> MWRKLLNNHHDDASKFICLLAKPNCSSLEQEDFIPLLQDVVDTHPGLTFLK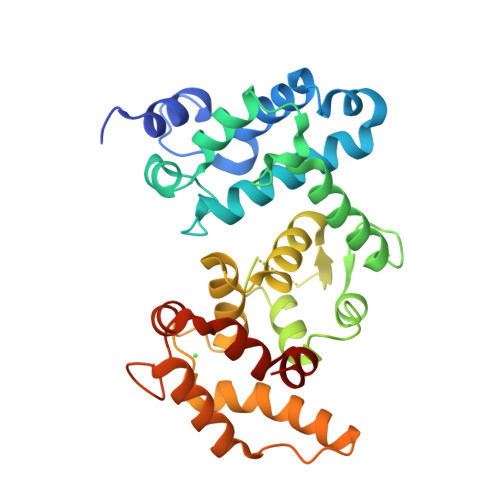DAPEFHSRYITTVIQRIFYTVNRSWSGKITSTEIRKSNFLQTLALLEEEEDINQITDYFSYEHFYVIYCKFWELDTDHDLYISQADLSRYNDQASSSRIIERIFSGAVTRGKTIQKEGRMSYADFVWFLISEEDKRNPTSIEYWFRCMDVDGDGVLSMYELEYFYEEQCERMEAMGIEPLPFHDLLCQMLDLVKPAVDGKITLRDLKRCRMAHIFYDTFFNLEKYLDHEQRDPF>[6x]MPGIRGPSEYSQEPPRHPSLKVNAKEPFNAEPPRSALVSSYVTPVDLFYKRNHGPIPIVDHLQSYSVTLTGLIQNPRKLFIKDIRSLPKYNVTATLQCAGNRRTAMSKVRNVRGVGWDVSAIGNAVWGGAKLADVLELVGIPKLTASTNLGARHVEFVSVDRCKEENGGPYKASITLSQATNPEADVLL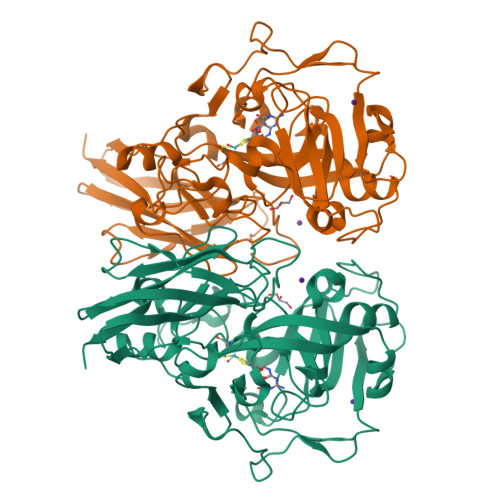AYEMNGETLNRDHGFPLRVVVPGVIGARSVKWLDSINVIAEESQGFFMQKDYKMFPPSVNWDNINWSSRRPQMDFPVQSAICSVEDVQMVKPGKVSIKGYAVSGGGRGIERVDISLDGGKNWVEASRTQEPGKQYISEHSSSDKWAWVLFEATIDVSQTTEVIAKAVDSAANVQPENVESVWNLRGVLNTSWHRVLLRLGHSNL Gene transfer agents (GTAs) are DNA-containing phage-like particles produced by some species of bacteria and archaea. The genes encoding proteins that form Rhodobacter capsulatus GTA particles (RcGTA) are derived from phage DNA, which has been integrated into the bacterial genome. Here, we use cryo-electron microscopy (cryo-EM) to determine the structures of RcGTA before and after DNA ejection, and to visualize the interactions of RcGTA with R. capsulatus cells. Particles of RcGTA have heads with a diameter of 38-nm and 49-nm long tails.

The asymmetric reconstruction of the native particle of RcGTA has an overall resolution of 4.3 Å, and symmetrized reconstructions of the head, portal complex, tail, and baseplate have resolutions of 3.3–4.5Å. Asymmetric reconstruction of the RcGTA particle at a resolution of 4.3 Å enabled characterization of the interface between the capsid and portal complex. Incorporation of the portal complex into the capsid is enabled by changes in the structure of the major capsid proteins relative to their structures in the rest of the capsid. Residues 99–106 from the N-termini of major capsid proteins interacting with the portal are tilted 18° away from the portal complex relative to their orientation in other capsid proteins. This conformational change enables the N-terminus to fit inside a groove formed by the wing domain of the portal complex and peripheral domain and extended loop of the capsid protein. The asymmetric reconstruction of the RcGTA particle shows that interactions of the capsid with portal and adaptor complexes induce deviations of the structures from their ideal fivefold and twelvefold symmetries, respectively. By contrast, an asymmetric reconstruction of the portal and adaptor complexes of RcGTA, determined to a resolution of 4.3 Å, does not show any unique interactions between the portal or adaptor proteins and the packaged DNA. Therefore, the DNA is probably held in the RcGTA head by the tape measure proteins and iris-like constriction within the baseplate, which block the tail channel. Furthermore, the end of the DNA packaged in the native RcGTA particle extends through the channel formed by the hexamer of stopper proteins and continues into the disc of tail terminator proteins.

>[12x]MGLNFFRKAAPEVRTEPVAERKASVTGRIVAMASGAGRPVWGPRDTVSLMRTGFAGNPVGFRSVKLIAEATAAVPLICQDAERRYEIHPVLDLLRRPNAGQGRAELFEALIGQILLSGNGYLEAVCPEPGVPRELHVLRSDRMAVVPGADGWPVGYDYTVGGRKHRFDMTGHPDPICHIKSFHPTDDHYGLSPMQAAAVALDVHNAASAWSKALLDNAARPSGAIIYKGADGQGVLAPEQYERLIFEMETHHQGARNAGRPMLLEGGLDWKPMGFSPSDMEFHETKAAAAREIALAFGVPPMLIGIPGDATYANYAEANRAFYRLTVLPLLTRVSAALAWWLSGYLGAQIELKPDLDQVPALAVERDQLWARIGAAGFLSNSEKRVLLGLPPTAEG;>MMLNEVTAVPGTALPVAEFRDHLRLGTGFADLGAEDAALLSYLRAAIAAIEGRTAKALISRGFRLALTAWRWGDMQTLPIAPVATVTALRLVDAAGVETPVAAGWRLVPDMARPRIEALGAMLPMIPTGGRVEIDFTAGFGASWSALPVDLAQAVFLLAAQYYELRHDGAAEGGAMPFGVMALIERWRTVRVLGGRP[12x];>MSRPRLNRLLVLEEAVRVADGAGGHRLDWQAKGEVWAEVTAGSGSERAGEFVTLASVPFTIVVRAAPVGAARRPRPEQRFREGARIFRILAVAERDREGHYLSCFAREEVVA[6x];>MSYAVAGALQAAVYQQLRADAVLAALVGTAVYDAVPPGPLAGTYVSLGPEDVADASDKTGAGAVHDFVISVITDAAGFATAKAAAAAVSDALVGADLVLSRGRLVGLWFLRAKARRVEKADMRRIDLVFRARVEG[6x];>[30x]MAAQNGKDLLIKLDLTGSGQFETIAGLRATRISFNAETVDVTSLESQGGWRELLGGAGVRSASISGAGVFKDADTDERARQIFFDGEVPEFQVIIPDFGIVQGPFMITSIDYAGSHNGEASYELAMASAGALSFTAI;>[6x]MAFHEVRFPANLSFGSVGGPERRTEIVTLSSGHEERNSPWAHSRRHYDAGVGLRSLDDVERLIAFFEARGGQLHGFRWKDWADFKSCPASRAVAHEDQLIGMGDGVTTAFQLVKTYVSGGQSYLRPIVKPVEGTVKLGIAGDHQAEAVNFAVDHATGIVSFNEPPPQGARVTAGFEFDVPVRFDTDRIAVSVQSFQAGDLPQVPVVEVRI;>[3x]MAYPESLKAHLQGGVTTLARAWALARADGRVLGFTDHDVVLRFDGISFEPGSGMTAKAVLQGTGLSVDNTESYGALSSEAITEADLLAGRYDGAAVTVWLVNWADPAMRAVIFRGHLGEVSRGAGAFTAELRGLTAALGQEQGRIYHPRCAAVLGDGRCRFDLTKDGYALEAALGGVDEAVVLRLAEGAGFEDRWFEKGRLVVLDGAAAGLIGVVKNDRLQADGSRLIELWQRLGANPVAGDRVRIEPGCDKRAGTCRLKFDNFLNFRGFPHIPGEDWMVSYPVQSGTNDGGSLFR;>[3x]MATILLSAAGAAIGGGFGGTVLGLSGAVIGRAVGATLGRVIDQRLLGSGSQSVETGRVDRLRLSSASEGEAVGRLWGRMRVAGQVIWATRFFESASVEKSGKGVPRATVTSYSYSLSLALALCEGEILRVGRVWADGSEIEVSGLNMRVYRGGEDQLPDPKIAAVEGAEAAPAYRGIAYVVLEDLQLAPFGNRVPQFTFEVVRAAQGALAEAEPDLTRGLRAVALIPGTGEYALATTPVYLATGSGVTATQGVANQNAPGGQTDLVAALERLDEELPNCGAVSLVVSWFGDDLRCGACDVKPKVASVAEEGANMPWRVAGLERAGAEEVPRLSGQSVYGGTPADAAVIEAIAALRAAGKAVTFYPFILMAQLAGNGLPDPWNPGSAQPALPWRGRITLSVAPGRAGSPDGTAAAEAQVAGFFGAASPGDSAIAGGEVVYSGPEEWSMRRFILHYAHLCQLAGGVDAFCIGTEMVALTQIRGPSNSFPAVAAFRQLAGEVKAILGPGCKIGYAADWSEYWGYAPGNGERFFHLDPLWADENIDFIGIDNYLPLSDWRDGADHADAGWGSIHALDYLRSNIEGGEYYDWFYAAPEHRAAQIRTPITDGDHDEPWIWRAKDLRNWWLNDHHERVGGLRSEVATAWVPQSKPIWFTEMGCAAIDKGTNQPNKFLDPKSSESGLPHHSDGRRDELIQMQYLRAMTGYWGEAARNPVSAVYGGPMLDMSRAHVWAWDARPWPQFPLNTALWSDGENYARGHWISGRAVAQPLASVVAEICGAAGITEIDVSGLYGLVRGYTMTGDQTGRAGLQALMLAYGFEALERDGQLVFRMRDGRVAADLAAADLALGEGEAVVETVRAAEAEIAGRVRLAYVEAEGDFEVKAVEAVFPDAAAGAAAGSELSLALTRAQAQGIVGRWLAEARVARDTARFALPPSRGHLGTGDVVRLDLPEGKRRYRIDRVEQAGLIQVEAVRVEPGIYAPADEVEDPASLRPFAAPVPVTAVFLDLPLMKGDEDPVAPHLAVTATPWPGTVAVWSSDEDAGYALNASLGTRAVIGQTLTPLFRARPGVWDRGAALRVRLASGALDSATAAKVLNGANAMAIGDGSSENWEVFQFAEAALVEGKIWDISLRLRGQLGTDALMPEVWPEGSVVVALNGAPEQILLPSAARGLARHYRIGAAVRSYDDPSFVHRIEAFAGAGLRPFSPCHLRAEPGASGWAFRWVRRTRIDGDSWQGYEVPLGETAELYLVRVLEGTAVKREVTVGEASWSYPAALQAADGIAGAFTLEVAQVSDVYGPGLAARITVGA;>[55x]MDVFAKHAVSLESPAVRHYEITPSDSTDLARRPRALRVQTGGTLVLRDETGITVTYTVFAGEILPVRPVRVLATGTTATAVGWE;>MPEGADPVAEVKTALAGFLKEVKGFQDDVKTRLQQQEERVTMLQTKTYAGRHALAAAATEEAPHQKAFAAYLRTGDDDGLRGLSLEGKALNSAVAAEGGYLVDPQTSETIRGVLRSTASLRQIASVVNVEATSFDVLVDKTDMGSGWASETAALSETATPQIDRITIPLHELAAMPKASQRLLDDSAFDIETWLANRIADKFARAEAAAFISGDGVDKPTGFLTKTKVANGAWAWGSLGYVATGAAGDFAAVNASDAVVDLVYALGAEYRANASFVMNSKTAGAVRKMKDADGRFLWADSLAAGEPARLMGYPVLIAEDMPDIAANAYAIAFGDFGNGYTIAERPDLRVLRDPFSAKPHVLFYASKRVGGDVSDFAAIKLLKFAA[145x];>MIALGLGLGLAANGGPALRRYAVNGVAPVAVLDFERHFLSHPLALTRATSATYADALRAVQTAPADTPRYDYSTGKRALLLEASATNLLPNSAQFEAASWGKTRASVLANAALAPNGTMTADKLVEDTSNNSHFVARTGTQIAAGTSVTASIFVKAAERRWFALVTADSANAFRTTYFDLQTGTLGVVSQGAAGHVAQIVAAGNGWYRCSVTQTQAASGNFNFYPSVASANGATSYPGDGASGLYLWGAQLEAGAAVSSVIPTEAAAVTRAADLASVAVAAGSYDLRRVDAAGTAVTKGVAHPGGALTIGAGSLYLLSLFPAGAL[10x]>[4x]HMSVGIVYGDQYRQLCCSSPKFGDRYALVMDLINAYKLIPELSRVPPLQWDSPSRMYEAVTAFHSTEYVDALKKLQMLHCEEKELTADDELLMDSFSLNYDCPGFPSVFDYSLAAVQGSLAAASALICRHCEVVINWGGGWHHAKRSEAS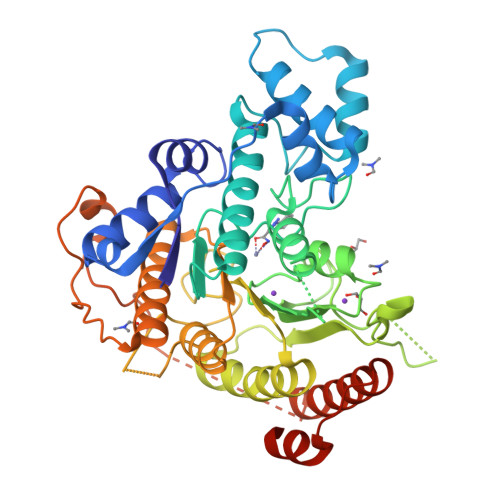GFCYLNDIVLAIHRLVSSTPPETSPNRQTRVLYVDLDLHHGDGVEEAFWYSPRVVTFSVHHASPGFFPGTGTWNMVDNDKLPIFLNGAGRGRFSAFNLPLEEGINDLDWSNAIGPILDSLNIVIQPSYVVVQCGADCLATDPHRIFRLTNFYPNLNLDSDCDSECSLSGYLYAIKKILSWKVPTLILGGGGYNFPDTARLWTRVTALTIEEVKGKKMTISPEIPEHSYFSRYGPDFELDIDYFPHESHNKTLDSIQKHHRRILEQLRNYADLNKLIYDYDQVYQLYNLTGMGSLVPR> QPQS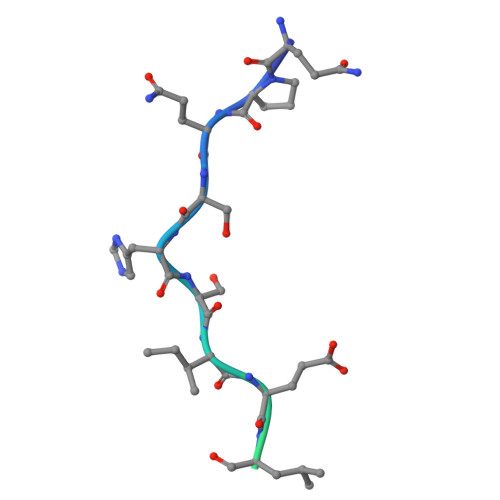HSIELDEVSKEAASTRAALTSNL>MIFVNDVYKNFGSLEVLKGVTLKVNKGEVVVIIGPSGSGKSTLLRCINLLEEPTKGEVFIDGVKINNGKVNINKVRQKVGMVFQHFNLFPHLTAIENITLAPVKVKKMNKKEAEELAVDLLAKVGLLDKKDQYPIKLSGGQKQRLAIARALAMQPEVMLFDEPTSALDPEMVKEVLNVMKQLANEGMTMVVVTHEMGFAREVGDRVIFMDDGVIVEEGTPEEIFYRAKNERTREFLSKIL[2x];>MTVDFLSMVKYTPLFISGLIMTLKLTFLAVTIGVLMGLFIALMKMSSIKPIKLVASSYIEVIRGTPLLVQLLLIYNGLMQFGMNIPAFTAGVSALAINSSAYVAEIIRAGIQAVDPGQNEAARSLGMTHAMAMRYVIIPQAIKNILPALGNEFIVMLKESAIVSVIGFADLTRQADIIQ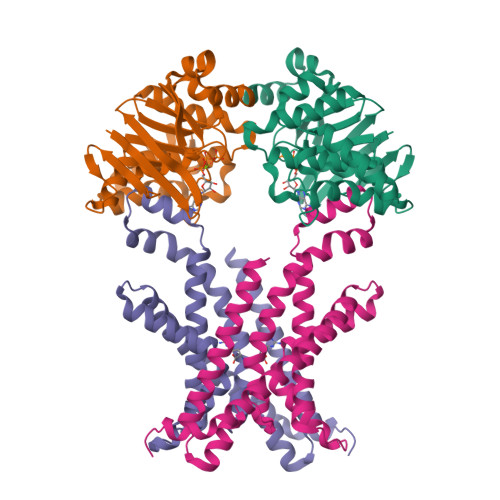SVTYRYFEPYIIIAAIYFVMTLTFSKLLSLFERRLRAGDIR[2x]PgcA has been shown to play an important role in EET but is unusual in containing three CXXCH heme binding motifs that are separated by repeated (PT)x motifs, suggested to enhance binding to mineral surfaces. The amino acid sequence of PgcA contains a cleavable Sec signal peptide followed by an N‐terminal lipid anchor and four domains interspersed by repeated (PT)x motifs. The first domain is not predicted to contain any cofactors, while the other three domains are monoheme domains (Fernandes et al., 2023). Furthermore, we demonstrate a distinct role for its domain III as a mineral reductase that is recharged by domains I and II. These findings show PgcA to be the first of a new class of electron transfer proteins, with redox centers separated by some nanometers but tethered together by flexible linkers, facilitating electron transfer through a tethered diffusion mechanism rather than a fixed, closely packed electron transfer chain.

The 1.8 Å crystal structure of heme domain II consisted of six copies of the protein within the asymmetric unit, comprising residues 352–414 of the PgcA amino acid sequence. The overall fold is the same within each copy and consists of four loop‐linked α‐helices encapsulating the c‐type heme moiety. The structures of domains I and II are highly similar, with a root mean square deviation (RMSD) of 0.453 Å and share 53% sequence identity. Like domain I, domain II displays His‐Met heme ligation (in this case from residues His365 and Met392) and the imidazole groups of His365 are within H‐bonding distance (2.7 Å) of the carboxylate group of Asp372. This suggests that PgcA domains I and II likely arose from a gene duplication event and that both the heme axial ligands and the histidine coordinated acidic residues are important structural features of these domains. Domains I and II possess two acidic residues, Glu281 and Asp372, which hydrogen bond the proximal histidine of the His–Met coordinated heme. These negatively charged residues might help stabilize the Fe3+ state over Fe2+, supported by the pH‐dependent voltammograms which show that these two domains have E m that is significantly more pH sensitive than domain III. From domain III to domain I to domain II, the spectra have increasingly anisotropic signatures where the g max value becomes more intense than the other two g‐values (De & Albracht, 1979) (g max = 3.23 and 3.37 for domain I and II, respectively). A highly anisotropic or axial LS (HALS) type “large g max” signal (g > 3.2) can occur when two histidine heme ligands are perpendicular to each other but is also typical of histidine–methionine heme coordination where ligand orientation cannot be resolved (Zoppellaro et al., 2009).

>[6x]MKFKLNLITLALLANTGLAVAADGNGSALYGNNCQACHGSITNSDIQTRTVSAIQSAISGNRGGMGFLSTLTSAEIQAIATSLASAVGSGWSHPQFEK>QTYTVSENKRFLLKDGKPFFWLGDTAWELFHRLDREDADYYLKKRAAQKYTVIQAVALAEFDGLNVPNPYGDKPLLNNDPTTPNDAYFKHVDFIIDKAAEYGLTIGFLPTWGDKLNKSTWGKGPEVFNTNNARIYGKWLANRYKNKKNIIWILGGDRTPRPNSDDVKVWRAMAAGIVEGVGGNDKALITFHPQPNKEGASQWFHADEWFDFNMFQNGHCRDTPIYDNIKGSYDRALVKPVIDGEPIYEDHPVCFNATDLGISNAYDVRKYAYLNLFAGAFGHTYGCHDIWQMYSPFREAVNGPNFYWQQAMELPGAKQMQHARKLIESRPFLDRVPDQSLVVENNSPASERIQATRGKDYAFIYSAAGKSFTVNLGKISGTQLNAYWFDPRNGKVEDISKIDNKGTYKFTPPRSGYGQDWVLILDDASKNFLKP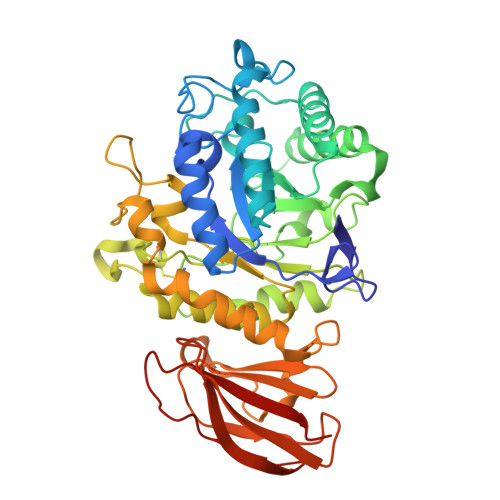[4x]> MEPHVLGAVLYWLLLPCALLAACLLRFSGLSLVYLLFLLLLPWFPGPTRCGLQGHTGRLLRALLGLSLLFLVAHLALQICLHIVPRLDQLLGPSCSRWETLSRHIGVTRLDLKDIPNAIRLVAPDLGILVVSSVCLGICGRLARNTRQSPHPRELDDDERDVDASPTAGLQEAATLAPTRRSRLAARFRVTAHWLLVAAGRVLAVTLLALAGIAHPSALSSVYLLLFLALCTWWACHFPISTRGFSRLCVAVGCFGAGHLICLYCYQMPLAQALLPPAGIWARVLGLKDFVGPTNCSSPHALVLNTGLDWPVYASPGVLLLLCYATASLRKLRAYRPSGQRKEAAKGYEARELELAELDQWPQERESDQHVVPTAPDTEADNCIVHELTGQSSVLRRPVRPKRAEPREASPLHSLGHLIMDQSYVCALIAMMVWSITYHSWLTFVLLLWACLIWTVRSRHQLAMLCSPCILLYGMTLCCLRYVWAMDLRPELPTTLGPVSLRQLGLEHTRYPCLDLGAMLLYTLTFWLLLRQFVKEKLLKWAESPAALTEVTVADTEPTRTQTLLQSLGELVKGVYAKYWIYVCAGMFIVVSFAGRLVVYKIVYMFLFLLCLTLFQVYYSLWRKLLKAFWWLVVAYTMLVLIAVYTFQFQDFPAYWRNLTGFTDEQLGDLGLEQFSVSELFSSILVPGFFLLACILQLHYFHRPFMQLTDMEHVSLPGTRLPRWAHRQDAVSGTPLLREEQQEHQQQQQEEEEEEEDSRDEGLGVATPHQATQVPEGAAKWGLVAERLLELAAGFSDVLSRVQVFLRRLLELHVFKLVALYTVWVALKEVSVMNLLLVVLWAFALPYPRFRPMASCLSTVWTCVIIVCKMLYQLKVVNPQEYSSNCTEPFPNSTNLLPTEISQSLLYRGPVDPANWFGVRKGFPNLGYIQNHLQVLLLLVFEAIVYRRQEHYRRQHQLAPLPAQAVFASGTRQQLDQDLLGCLKYFINFFFYKFGLEICFLMAVNVIGQRMNFLVTLHGCWLVAILTRRHRQAIARLWPNYCLFLALFLLYQYLLCLGMPPALCIDYPWRWSRAVPMNSALIKWLYLPDFFRAPNSTNLISDFLLLLCASQQWQVFSAERTEEWQRMAGVNTDRLEPLRGEPNPVPNFIHCRSYLDMLKVAVFRYLFWLVLVVVFVTGATRISIFGLGYLLACFYLLLFGTALLQRDTRARLVLWDCLILYNVTVIISKNMLSLLACVFVEQMQTGFCWVIQLFSLVCTVKGYYDPKEMMDRDQDCLLPVEEAGIIWDSVCFFFLLLQRRVFLSHYYLHVRADLQATALLASRGFALYN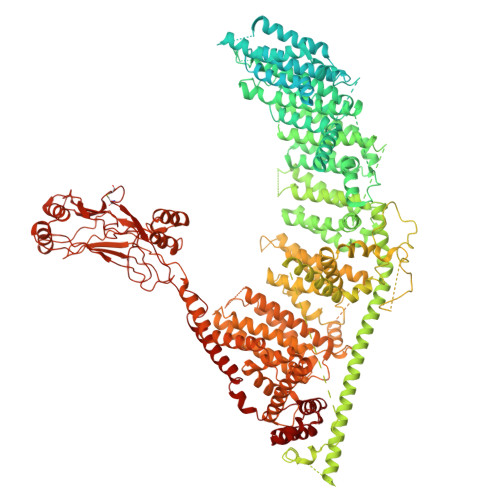AANLKSIDFHRRIEEKSLAQLKRQMERIRAKQEKHRQGRVDRSRPQDTLGPKDPGLEPGPDSPGGSSPPRRQWWRPWLDHATVIHSGDYFLFESDSEEEEEAVPEDPRPSAQSAFQLAYQAWVTNAQAVLRRRQQEQEQARQEQAGQLPTGGGPSQEVEPAEGPEEAAAGRSHVVQRVLSTAQFLWMLGQALVDELTRWLQEFTRHHGTMSDVLRAERYLLTQELLQGGEVHRGVLDQLYTSQAEATLPGPTEAPNAPSTVSSGLGAEEPLSSMTDDMGSPLSTGYHTRSGSEEAVTDPGEREAGASLYQGLMRTASELLLDRRLRIPELEEAELFAEGQGRALRLLRAVYQCVAAHSELLCYFIIILNHMVTASAGSLVLPVLVFLWAMLSIPRPSKRFWMTAIVFTEIAVVVKYLFQFGFFPWNSHVVLRRYENKPYFPPRILGLEKTDGYIKYDLVQLMALFFHRSQLLCYGLWDHEEDSPSKEHDKSGEEEQGAEEGPGVPAATTEDHIQVEARVGPTDGTPEPQVELRPRDTRRISLRFRRRKKEGPARKGAAAIEAEDREEEEGEEEKEAPTGREKRPSRSGGRVRAAGRRLQGFCLSLAQGTYRPLRRFFHDILHTKYRAATDVYALMFLADVVDFIIIIFGFWAFGKHSAATDITSSLSDDQVPEAFLVMLLIQFSTMVVDRALYLRKTVLGKLAFQVALVLAIHLWMFFILPAVTERMFNQNVVAQLWYFVKCIYFALSAYQIRCGYPTRILGNFLTKKYNHLNLFLFQGFRLVPFLVELRAVMDWVWTDTTLSLSSWMCVEDIYANIFIIKCSRETEKKYPQPKGQKKKKIVKYGMGGLIILFLIAIIWFPLLFMSLVRSVVGVVNQPIDVTVTLKLGGYEPLFTMSAQQPSIIPFTAQAYEELSRQFDPQPLAMQFISQYSPEDIVTAQIEGSSGALWRISPPSRAQMKRELYNGTADITLRFTWNFQRDLAKGGTVEYANEKHMLALAPNSTARRQLASLLEGTSDQSVVIPNLFPKYIRAPNGPEANPVKQLQPNEEADYLGVRIQLRREQGAGATGFLEWWVIELQECRTDCNLLPMVIFSDKVSPPSLGFLAGYGIMGLYVSIVLVIGKFVHGFFSEISHSIMFEELPCVDRILKLCQDIFLVRETRELELEEELYAKLIFLYRSPETMIKWTREKE> REFTIDFSTQQSYVSSLNSIRTEISTPLEHISQGTTSVSVI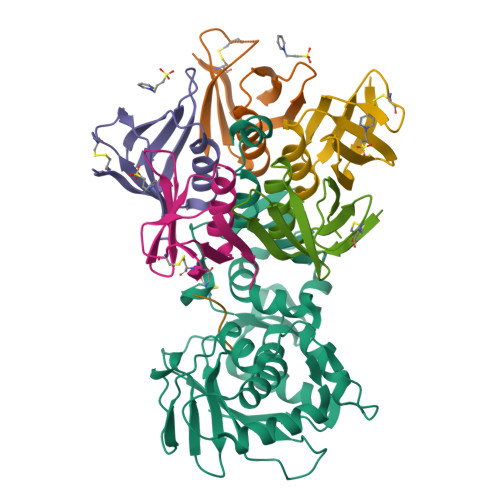NHTPPGSYFAVDIRGLDVYQARFDHLRLIIEQNNLYVAGFVNTATNTFYRFSDFTHISVPGVTTVSMTTDSSYTTLQRVAALERSGMQISRHSLVSSYLALMEFSGNTMTRDASRAVLRFVTVTAEALRFRQIQREFRQALSETAPVYTMTPGDVDLTLNWGRISNVLPEYRGEDGVRVGRISFNNISAILGTVAVILNCHHQGARSVRAVNEESQPECQITGDRPVIKINNTLWESNTAAAFLNRKSQFLYTTGK;>ADCAKGKIEFSKYNEDDTFTVKVDGKEYWTSRWNLQPLLQSAQLTGMTVTIKSSTCESGSGFAEVQFNND[5x];> ARRRRAX2-methyl-4-{4-[2-(morpholin-4-yl)-2-oxoethyl]phenoxy}benzonitrile | C20 H20 N2 O3 | 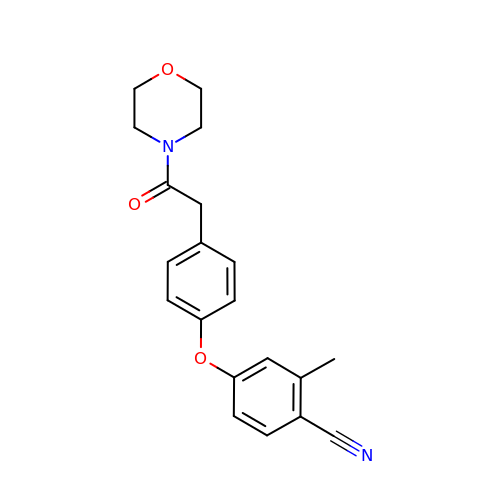QOJWBEUMAJACBY-UHFFFAOYSA-N>MGSDKIHHHHHHMFDPESLKKLAIEIVKKSIEAVFPDRAVKETLPKLNLDRVILVAVGKAAWRMAKAAYEVLGKKIRKGVVVTKYGHSEGPIDDFEIYEAGHPVPDENTIKTTRRVLELVDQLNENDTVLFLLSGGGSSLFELPLEGVSLEEIQKLTSALLKSGASIEEINTVRKHLSQVKGGRFAERVFPAKVVALVLSDVLGDRLDVIASGPAWPDSSTSEDALKVLEKYGIETSESVKRAILQETPKHLSNVEIHLIGNVQKVCDEAKSLAKEKGFNAEIITTSLDCEAREAGRFIASIMKEVKFKDRPLKKPAALIFGGETVVHVKGNGIGGRNQELALSAAIALEGIEGVILCSAGTDGTDGPTDAAGGIVDGSTAKTLKAMGEDPYQYLKNNDSYNALKKSGALLITGPTGTNVNDLIIG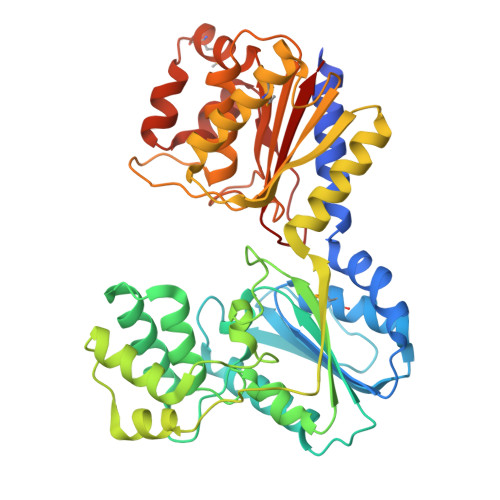LIV[2x]a type I PDZ binding motif (PBM). proteins are widely considered to act as scaffold proteins. activation through intranuclear sequestration and subsequent degradation. assay confirms that HN12-NS1 and PDlim2 interact in vitro.

PDZ-peptide complex either by soaking or co-crystallization. Ribbon diagram of two adjacent PDlim2 PDZ-hexapeptide fusion proteins. hexapeptide, and the comparison with similar structures. good model to investigate the binding mechanism between PDZ domains and the NS1 PBM. HN12-NS1 are crucial for their binding interaction. of the two basic residues (Arg16 and Lys31) in the PDlim2 PDZ domain. compromising the binding between the RSEV PBM and the PDlim2 PDZ domain. residue is a critical site for the binding selectivity of PDlim2. PDlim2, the Ser residues may allow the special selectivity to the NS1 (ESEV). residue to Arg16 of PDlim2 is strictly conserved in all of these proteins.

> MALTVDVAGPAPWGFRITGGRDFHTPIMVTKVAERGKAKDADLRPGDIIVAINGESAEGMLHAEAQSKIRQSPSPLRLQLDRSTIESEV> TTQKKVVLSSFSIIGDITQNIAKDLVTVTTLVEAGNDSHSYQVTSADAIKIQNADLILCNGLHLEETFMKYFTNLKKGTKIITVTDGINPIGVSEDTSVDSEPNPHAWMSLTNAMIYIENIRKALTALDPSNAKKYELNAREYSEKIRNSILPLKTRIEKVDPEKRWFVTSEGCLVYLAEDFGFKSLYLWPINSDSERSPSMMRHAINQMRSHKIKFIFSESTNSDQPAKQVAYETNASYGGVLYVDSLSK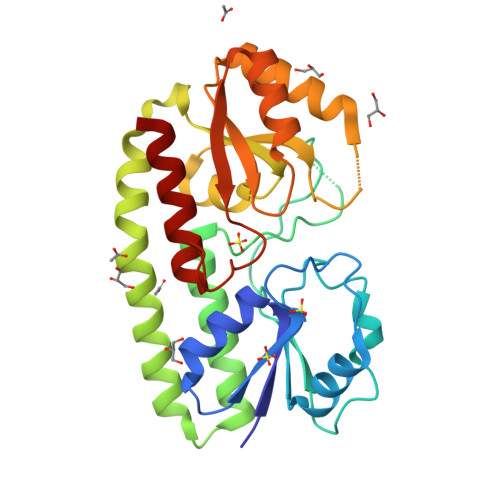PDGPAPTYLDLLRFSLTKIVDTLF>[4x]SNAMKAPELQIQQWFNSATDLTLADLRGKVIVIEAFQMLCPGCVMHGIPLAQKVRAAFPEDKVAVLGLHTVFEHHEAMTPISLKAFLHEYRIKFPVGVDQPGDGAMPRTMAAYQMR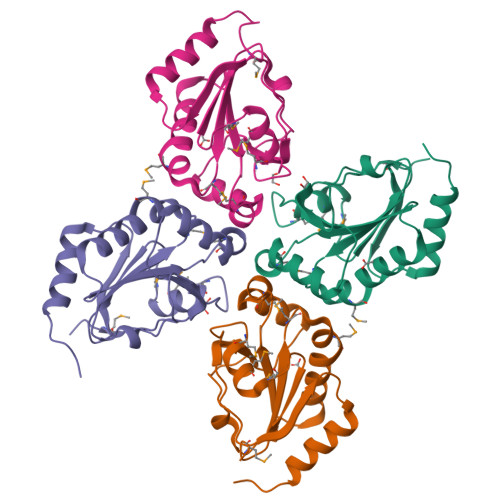GTPSLLLIDKAGDLRAHHFGDVSELLLGAEIATLLGEAAPSV> GPLGSMVATVKRTIRIKTQQHILPEVPPVENFPVRQWSIEIVLLDDEGKEIPATIFDKVIYHLHPTFANPNRTFTDPPFRIEEQGW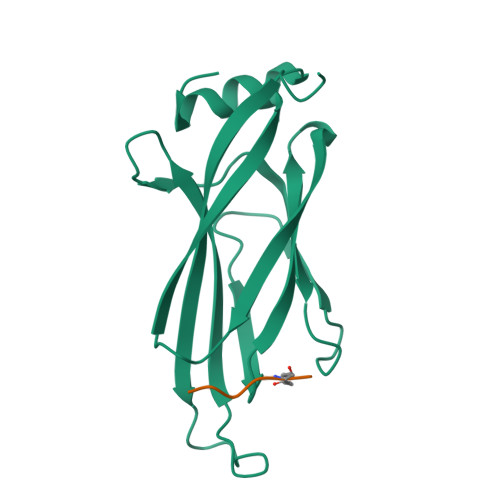AGFPLDISVFLLEKAGERKIPHDLNFLQESYEVEHVIQIPLNKPLLTEELAKSGST> MSSFYTVVGVFIVVSAMSVLFWIMAPKNNQAVW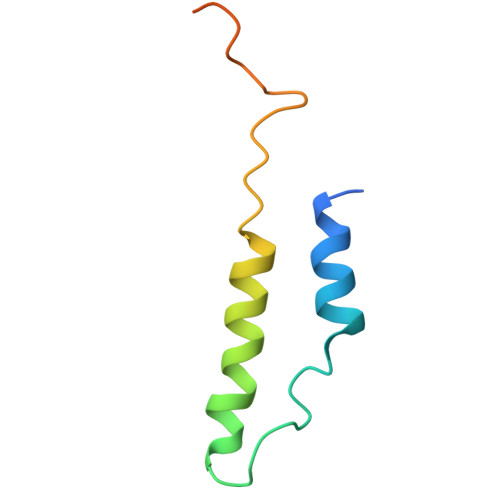RSTVILTLAMMFLMWAITFLCQLHPLVAPRRSDLRPEFAE Synaptotagmins (SYTs) are the plant orthologous of E-Syts and regulate the ER–PM communication in response to abiotic stress. In vivo studies showed that SYT1 is anchored to the ER through an N-terminal hydrophobic region and binds to the PM through the two C2 domains at the C-terminal end. Similar to other C2 domains, SYT1C2A folds as a four-stranded β sandwich with a Ca2+-binding site placed in a cavity formed by three loops connecting the two sheets (L1, L2, and L3). We have shown that the domain displays a dual activity to bind PS or PIPs in a Ca2+-dependent or independent manner, respectively.

Unexpectedly, we were able to solve the structure of SYT1C2A with one cadmium ion (Cd2+) at site II using different crystallization conditions. This structure mimics that with one Ca2+ at the high-affinity binding site. Indeed, the analysis of oxygen, Ca2+, and Cd2+ complexes found in the Cambridge Structural Database of chemical structures determined at high resolution reveals that the coordination numbers and geometries of Ca2+ and Cd2+ with oxygens are very similar. Interestingly, the comparative analysis of the structures of SYT1C2A in complex with Ca2+ and Cd2+ shows that Glu 334 at L3 changes its conformation to replace a water molecule at site II, whereas the positively charged side chain of Lys 275 replaces the Ca I. In this conformation, SYT1C2A might be unable to bind membranes through this site as Ca II would be occluded to interact with the phosphate moiety of phospholipids. Thus, these data might provide the structural basis for Ca2+-mediated activation of SYT1C2A to bind membranes. The metal binding site of SYT1C2A restricts the metal–metal distance to 3.7 Å. Hence, it is likely that the constraints imposed at SYT1C2Asite hinders the presence of two Cd atoms site hinders the presence of two Cd atoms.

> KAFRRPVGIVHVKVVRAVGLRKKDLMGGADPFVKIKLSEDKIPSKKTTVKHKNLNPEWNEEFKFSVRDPQTQVLEFSVYDWEQVGNPEKMGMNVLALKEMVPDEHKAFTLELRKTLDGGEDGQPPDKYRGKLEVELLYKPFTEEE>IVGGYTCGANTVPYQVSLNSGYHFCGGSLINSQWVVSAAHCYKSGIQVRLGEDNINVVEGNEQFISASKSIVHPSYNSETYNNDIMLIKLKSAASLNSRVASISLPTSCASAGTQCLISGWGNTKSSGTSYPDVLKCLKAPILSDSSCKSASSFIITSNMFCAGYLEGGKDACQG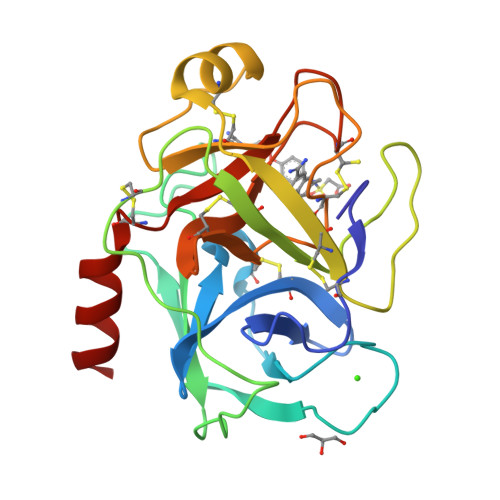DSGGPVVCSGKLQGIVSWGSGCAQKNKPGFYTKLCNYVSWIKQTIASN[2x]>[2x]GANAMGVLISAVGDTDPFRNFHDGALIHIARKYRPEKVILIFSEHTAKKQGNIEKALFSIAPNYEPELIIHDPIISDNEVHIFDVMFQRFSDILQEYYTKEDEFILNLSSATPQIKSALFVIN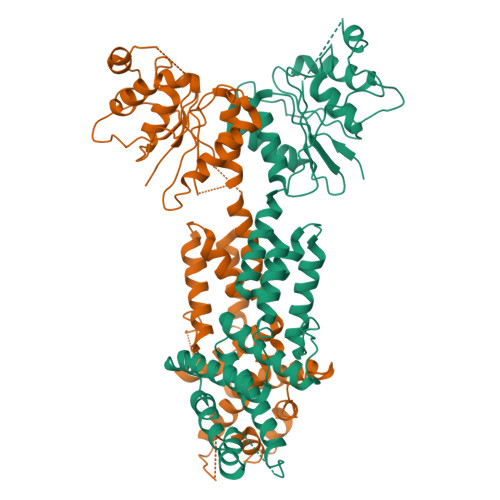RLNGINVKAVQVSSPEHASNENIGHDNDENIDELIEVNKDNKVNFIDRTIEDNAEKFSQALLKKTARDFIEKFDYKAALDILDQLSDFPNLKSVREEIRDVVNCLSKQDVPKGLRHKKLKEEEQKILSAYLTIELQRERGNVSESFIRIKNLTEFILEDYIKKRYPGLIDEYCEDIQKYYLSLFDYSKLLKATKEFKLKRTIAPIIDMNSSRNKVAHSLSPLDSDAVKQLGIAMKTLKTLVREQYHFSQSDFNFYQDLNKILLTKLN>MGSSHHHHHHSQDPGPENNLYSQYEQKVRPCIDLIDSLRALGVEQDLALPAIAVIGDQSSGKSSVLEALSGVALPRGSGIVTRCPLVLKLKKQPCEAWAGRISYRNTELELQDPGQVEKEIHKAQNVMAGNGRGISHELISLEITSPEVPDLTIIDLPGITRVAVDNQPRDIGLQIKALIKKYIQRQQTINLVVVPCNVDIATTEALSMAHEVDPEGDRTIGILTKPDLMDRGTEKSVMNVVRNLTYPLKKGYMIVKCRGQQEITNRLSLAEATKKEITFFQTHPYFRVLLEEGSATVPRLAERLTTELIMHIQKSLPLLEGQIRESHQKATEELRRCGADIPSQEADKMFFLIEKIKMFNQDIEKLVEGEEVVRENETRLYNKIREDFKNWVGILATNTQKVKNIIHEEVE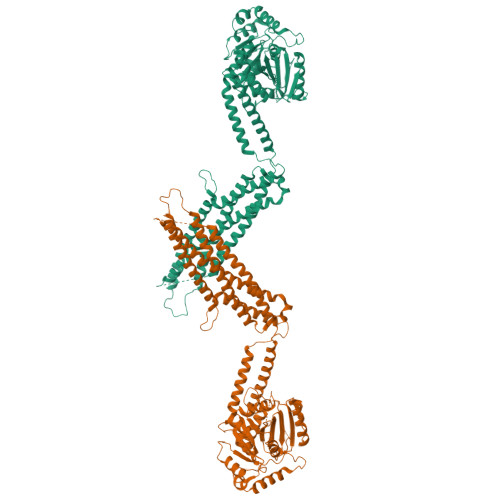KYEKQAAAAELLGFVNYKTFEIIVHQYIQQLVEPALSMLQKAMEIIQQAFINVAKKHFGEFFNLNQTVQSTIEDIKVKHTAKAENMIQLQFRMEQMVFCQDQIYSVVLKKVREEIFNPLGTPSQNMKLNSHFPSNESSVSSFTEIGIHLNAYFLETSKRLANQIPFIIQYFMLRENGDSLQKAMMQILQEKNRYSWLLQEQSETATKRRILKERIYRLTQARHALCQFSSKEIH[2x]> AADSARSFLERLEARGGREGAVLAGEFSDIQACSAAWKADGVCSTVAGSR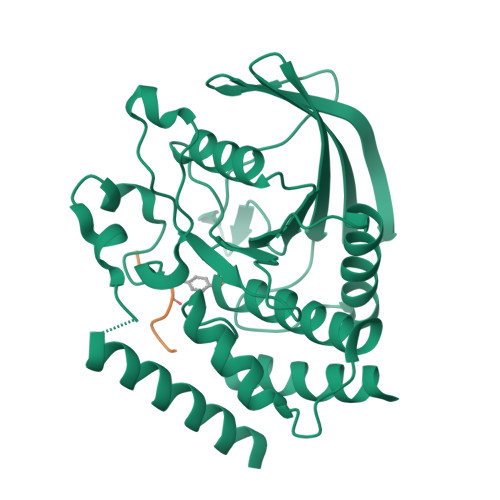PENVRKNRYKDVLPYDQTRVILSLLQEEGHSDYINGNFIRGVDGSLAYIATQGPLPHTLLDFWRLVWEFGVKVILMACREIENGRKRCERYWAQEQEPLQTGLFCITLIKEKWLNEDIMLRTLKVTFQKESRSVYQLQYMSWPDRGVPSSPDHMLAMVEEARRLQGSGPEPLCVHSSAGCGRTGVLCTVDYVRQLLLTQMIPPDFSLFDVVLKMRKQRPAAVQTEEQYRFLYHTVAQMFCSTLQNAS;> PEYLGLD>MGSSHHHHHHSAGENLYFQGTLPRETDEEPEEPGRRGSFVEMVDNLRGKSGQGYYVEMTVGSPPQTLNILVDTGSSNFAVGAAPHPFLHRYYQRQLSSTYRDLRKGVYVPYTQGKWEGELGTDLVSIPHGPNVTVRANIAAITESDKFFINGSNWEGILGLAYAEIARPDDSLEPFFDSLVKQTHVPNLFSLQLCGAGFPLNQSEVLASVGGSMIIGGIDHSLYTGSLWYTPIRREWYYEVIIVRVEINGQDLKMDCKEYNYDKSIVDSGTTNLRLPKKVFEAAVKSIKAASSTEKFPDGFWLGEQLVCWQAGTTPWNIFPVISLYLMGEVTNQSFRITILPQQYLRPVEDVATSQDDCYKFAISQSSTGTVMGAVIMEGFYVVFDRARKRIGFAVSAC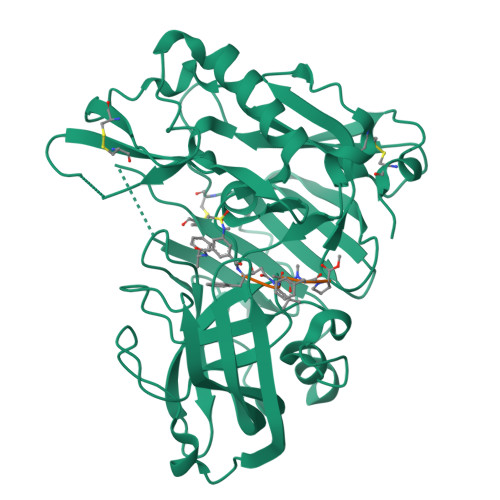HVHDEFRTAAVEGPFVTLDMEDCGYNIPQTDEST[3x]S-SAD phasing was applied to determine the structure of the N-terminal domain of the ectodomain of Hepatitis C virus envelope glycoprotein E1 (HCV nE1). The HCV envelope glycoproteins E1 and E2 are located on the surface of the virions and are responsible for binding of the virus to the host cells and membrane fusion. Although HCV is a major global health problem, its mechanism of fusion is still not known owing to the lack of structural knowledge of these two glycoproteins.

Here, the data collection and structure solution of the N-terminal domain of the ectodomain of HCV E1 from crystals that diffracted very weakly is reported. HCV nE1 is composed of 79 residues and contains no methionines, which makes this construct unsuitable for SeMet phasing. Heavy-atom soaking experiments were attempted but failed to show any useful anomalous signal for substructure determination; therefore, efforts were focused on S-SAD methods. By combining the data from 32 crystals, it was possible to solve the sulfur substructure and calculate initial maps at 7 Å resolution, and after density modication and phase extension using a higher resolution native data set to 3.5 Å resolution model building was achievable. The work reported here shows that useful phasing can be obtained without the need for high-resolution diffraction, or indeed strongly diffracting crystals, if careful data collection is carried out in order to obtain a highly redundant data set from mutiple crystals; indeed, the useful anomalous signal of HCV nE1 crystals did not extend to better than 6.5 Å resolution. The nature of the crystals is also very important; in our case we benefitted from isomorphous crystals, facilitating the scaling and merging of the data, whilst a high solvent content and NCS improved the quality of the early maps.

>ETGYQVRNSSGLYHVTNDCPNSSVVYEAADAILHTPGCVPCVREGQASRCWVAVTPTVATRDGKLPTTQLRRHIDLLVGSATENLYFQ[6x]>GIDPFTMQVSQYLYQNAQSIWGDCISHPFVQGIGRGTLERDKFRFYIIQDYLFLLEYAKVFALGVVKACDEAVMREFSNAIQDILNNEMSIHNHYIRELQITQKELQNACPTLANKSYTSYMLAEGFKGSIKEVAAAVLSCGWSYLVIAQNLSQIPNALEHAFYGHWIKGYSSKEFQACVNW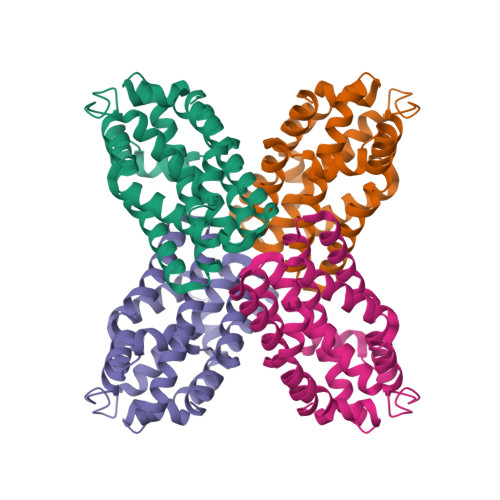NINLLDSLTLASSKQEIEKLKEIFITTSEYEYLFWDMAYQS[2x]(1R,3R)-5-((Z)-2-((1R,7AS)-HEXAHYDRO-1-((S)-6-HYDROXY-6-METHYLHEPT-4-YN-2-YL)-7A-METHYL-1H-INDEN-4(7AH)-YLIDENE)ETHYLIDENE)CYCLOHEXANE-1,3-DIOL 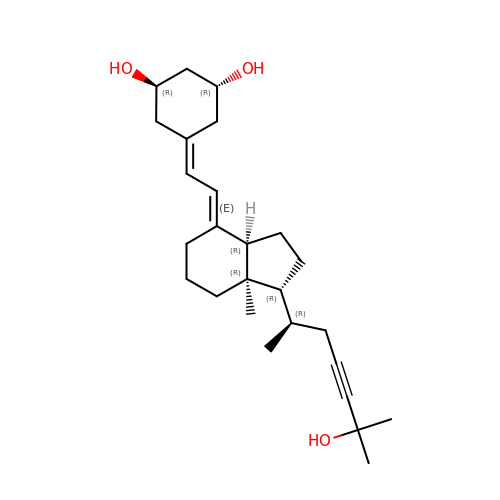| C26 H40 O3 | HHGRMHMXKPQNGF-XHJOVPLKSA-N> MGSDKIHHHHHHMTTIPSTAEAKLEMLTTINRAIAGSRPEALPPYPVPAPLSRAEILHQFEDRILDYGAAYTHVSAAELPGAIAKALGNARRVIVPAGIPAPWLTVGMDVLRDEPPLSHAELDRADAVLTGCAVAISETGTIILDHRADQGRRALSLIPDFHICVVREDQIVQTVREGVE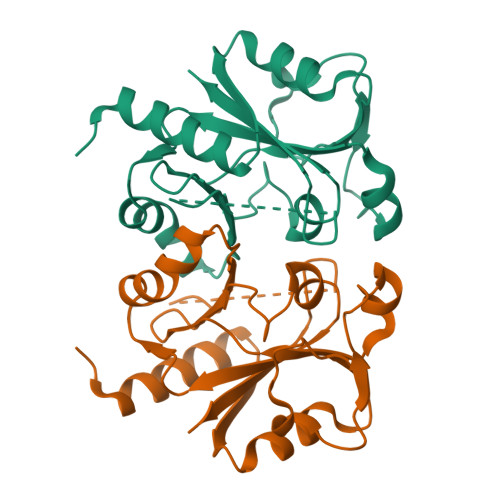AVAASVREGRPLTWLSGGSATSDIELVRVEGVHGPRRLQVIVVG>[2x]AYRDQPLGELALSIPRASALFRKYDMDYAAGGKQTLARAAARKELDVEVIEAELAKLAEQPIEKDWRSAPLAEIIDHIIVRYHDRHRE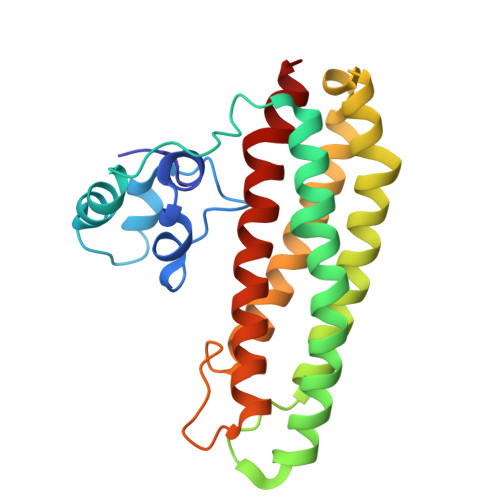QLPELILQATKVERVHADKPSVPKGLTKYLTMLHEELSSHMMKEEQILFPMIKQGMGSQAMGPISVMESLHDEAGELLEVIKHTTNNVTPPPEACTTWKAMYNGINELIDDLMDHISLENNVLFPRALAGE>GAELPAPLRRTGVGEWLATTCQGCTSWCAKQIYVMDGRALKVRGNPNSGVHGMSSCPRQHLSLQQVYDPDRLRTPMMRTNPKKGRDQDPKFVPISWDKALDMLADKIIALRVANEPHKYALLRGRYSHINDLLYKKMTNLIGSPNNISHSSVCAEAHKMGPYYLDGNWGYNQYDVKNAKFILSFGADPIASNRQVSFYSQTWGDSLDHAKVVVVDPRLSASAAKAHKWIPIEPGQDSVLALAIAHVALVEGVWHKPFVGDFIEGKNLFKAGKTVSVESFKETHTYGLVEWWNQALKDYTPEWASKITGIDPKTIIAIAKDMGAAAPAVQVWTSRGAVMQARGTYTSISCHALNGLFGGIDSKGGLFPGNKTPLLKEYPEAKAYMDEIAAKGVKKEKIDQRGRLEFPALAKGKSGGGVITANAANGIRNQDPYEIKVMLAYFNNFNFSNPEGQRWDEALSKVDFMAHITTNVSEFSWFADVLLPSSHHMFEKWGVLDSIGNGVAQISIQQPSIKRLWDTRIDESEIPYMLAKKLADKGFDAPWRYINEQIVDPETGKPAADEAEFAKLMVRYLTAPLWKEDASKYGDKLSSWDEFVQKGVWNSSPYKLEARWGKFKTETTKFEFYSKTLEKALQSHADKHKVSIDEVMKACDYQARGHLAFIPHYEEPYRFGDESEFPLLLVDQKSRLNKEGRTANSPWYYEFKDVDPGDVANEDVAKFNPIDGKKFGLKDGDEIRITSPVGMLTCKAKLWEGVRPGTVAKCFGQGHWAYGRYASAKFGVTPRGGSNNDLIADRYDRLSGASAFYGHIRVRVEKV[2x];>[2x]MRLGMVIDLQKCVGCGGCSLACKTENNTNDGIHWSHHIATTEGTFPDVKYTYIPTLCNHCDDAPCVKVCPT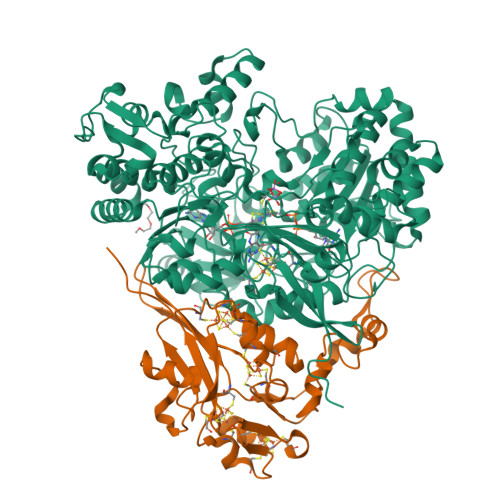GAMHKDKRGLTLQNNDECIGCKKCMNACPYGVISFNAATPHRRWQDDSEVVANGTVSPLMLLKRTGATATPNENPERGDTYPMIRPKRTTEKCTFCDHRLDKGLNPACVDACPSEARVIGDLDDPQSKVSQLIKLHKPMQLKPEAGTGPRVFYIRSFGVKTAY> QATNLAANLSAVRESATATLSGEIKGPQLEDFPALIKQASLDALFKCGKDAEALKEVFTNSNNVAGKKAIMEFAGLFRSALNATSDSPEAKTLLMKVGAEYTAQI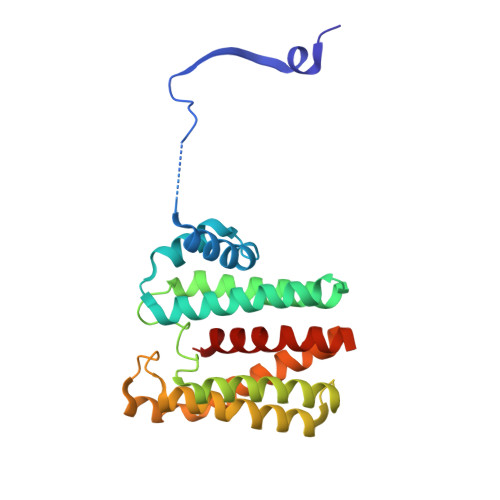IKDGLKEKSAFGPWLPETKKAEAKLENLEKQLLDIIKNNTGGELSKLSTNLVMQEVMPYIASCIEHNFGCTLDPLTRSNLTHLVDKAAAKAVEALDMCHQKLTQEQGTSVGREARHLEMQTLIPLLLRNVFAQIP5-FLUOROURIDINE | C9 H11 F N2 O6 | 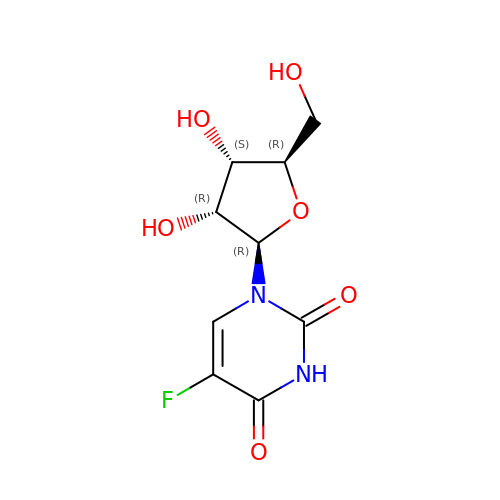FHIDNBAQOFJWCA-UAKXSSHOSA-N> ASWSHPQFEKGAELPVQRWWHKG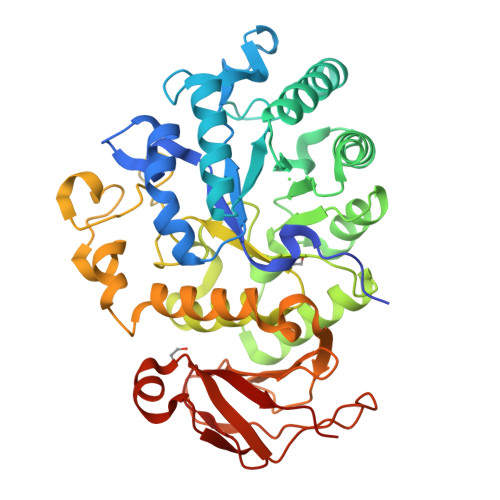ALYRIGDLQAFVGRDAGGIAGLKSHLEYLSTLKVKGLVLGPIHKNQKDEINETDLKQINPTLGSQEDFKDLLQSAKKKSIHIILDLTPNYQGQNAWFLPAQADIVATKMKEALSSWLQDGVDGFQFRDVGKLMNAPLYLAEWQNITKNLSEDRLLIAGTESSDLQQIVNILESTSDLLLTSSYLSNSTFTGERTESLVTRFLNATGSQWCSWSVSQAGLLADFIPDHLLRLYQLLLFTLPGTPVFSYGDELGLQGALPGQPAKAPLMPWNESSIFHIPRPVSLNMTVKGQNEDPGSLLTQFRRLSDLRGKERSLLHGDFHALSSSPDLFSYIRHWDQNERYLVVLNFRDSGRSARLGASNLPAGISLPASAKLLLSTDSARQSREEDTSLKLENLSLNPYEGLLLQFPFVA>MPGEIRPTIGQQMETGDQRFGDLVFRQLAPNVWQHTSYLDMPGFGAVASNGLIVRDGGRVLVVDTAWTDDQTAQILNWIKQEINLPVALAVVTHAHQDKMGGMDALHAAGIATYA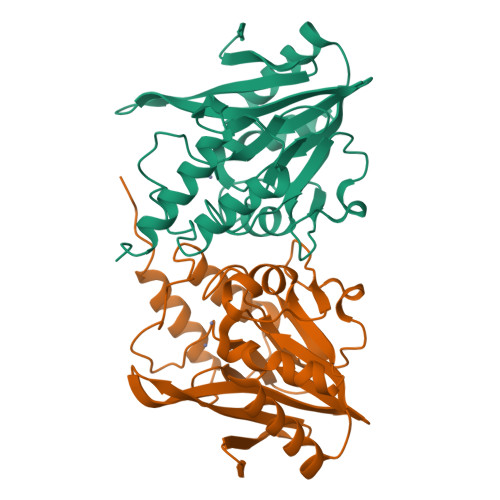NALSNQLAPQEGMVAAQHSLTFAANGWVEPATAPNFGPLKVFYPGPGHTSDNITVGIDGTDIAFGGCLIKDSKAKSLGNLGDADTEHYAASARAFGAAFPKASMIVMSHSAPDSRAAITHTARMADKLRKLVPRGSAAAALEHHHHHHHH[5x]>MFAKATRNFLREVDADGDLIAVSNLNDSDKLQLLSLVTKKKRFWCWQRPKYQFLSLTLGDVLIEDQFPSPVVVESDFVKYEGKFANHVSGTLETALGKVKLNLGGSSRVESQSSFGTLRKQEVDLQQLIRDSAERTINLRNPVLQQVLEGRNEVLCVLTQKITT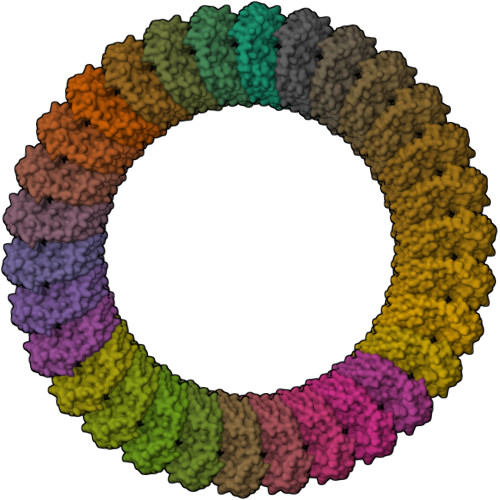MQKCVISEHMQVEEKCGGIVGIQTKTVQVSATEDGNVTKDSNVVLEIPAATTIAYGVIELYVKLDGQFEFCLLRGKQGGFE[30x]>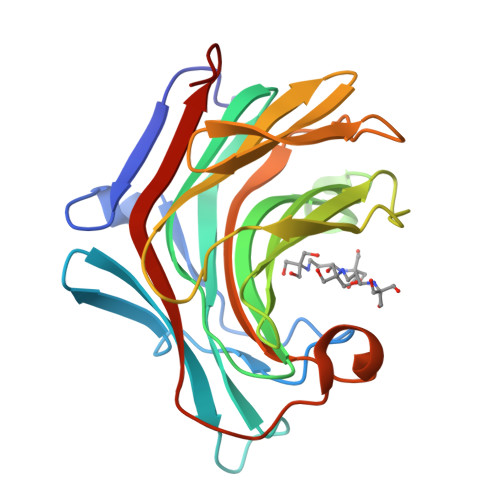[2x]ATVVNTPFVAVFSNFDSSQWEKADWANGSVFNCVWKPSQVTFSNGKMILTLDREYGGSYPYKSGEYRTKSFFGYGYYEVRMKAAKNVGIVSSFFTYTGPSDNNPWDEIDIEFLGKDTTKVQFNWYKNGVGGNEYLHNLGFDASQDFHTYGFEWRPDYIDFYVDGKKVYRGTRNIPVTPGKIMMNLWPGIGVDEWLGRYDGRTPLQAEYEYVKYYPNGVPQ> MADLHIGNYRLLKTIGKGNFAKVKLARHILTGKEVAVKIIDKTQLNSSSLQKLFREVRIMKVLNHPNIVKLFEVIETEKTLYLVMEYASGGEVFDYLV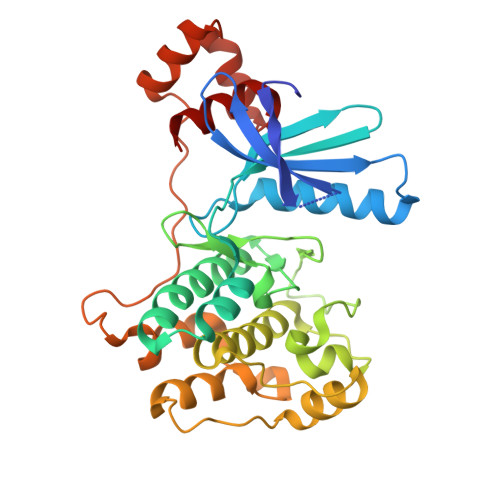AHGWMKEKEARAKFRQIVSAVQYCHQKFIVHRDLKAENLLLDADMNIKIADFGFSNEFTFGNKLDTFCGSPPYAAPELFQGKKYDGPEVDVWSLGVILYTLVSGSLPFDGQNLKELRERVLRGKYRIPFYMSTDCENLLKKFLILNPSKRGTLEQIMKDRWMNVGHEDDELKPYVEPLPDYKDPRRTELMVSMGYTREEIQDSLVGQRYNEVMATYLLLGY>SNAMETFLFTSESVNEGHPDKLCDQISDAVLDACLEQDPDSKVACETCTKTNMVMVFGEITTKATIDYEKIVRDTCRSIGFISDDVGLDADKCKVLVNIEQQSPDIAQGVHGHFTKRPEDIGAGDQGHMFGYATDETPELMPLSHVLATKIGARLTEVRKNGTCRWLRPDGKTQVTV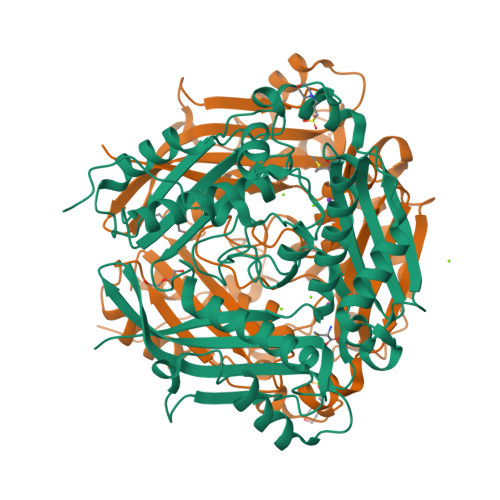EYYNDNGAMVPVRVHTVLISTQHDETVTNDEIARDLKEHVIKPIIPEKYLDDKTIFHLNPSGRFVIGGPHGDAGLTGRKIIIDTYGGWGAHGGGAFSGKDPTKVDRSGAYIVRQAAKSVVANGMARRALVQVSYAIGVPEPLSVFVDTYGTGLIPDKEILKIVKETFDFRPGMMTINLDLKRGGNGRFQKTAAYGHFGRDDPDFTWEVVKPLKWDKPQLNNIGSG[4x]>SNADEVQVAVAANFTAPIQAIAKEFEKDTGHRLVAAYGATGQFYTQIKNGAPFQVFLSADDSTPAKLEQEGEVVPGSRFTYAIGTLALWSPKAGYVDAEGEVLKSGSFRHLSIANPKTAPYGLAATQAMDKLGLAATLGPKLVEGQNISQAYQFVSSGNAELGFVALSQIYK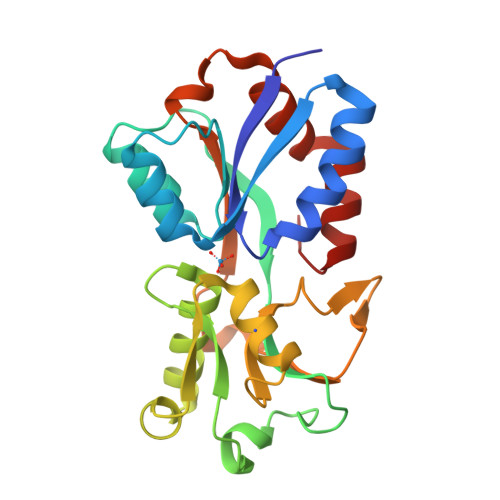DGKVATGSAWIVPTELHDPIRQDAVILNKGKDNAAAKALVDYLKGAKAAALIKSYGYEL[2x]> SDILGMLKSLHQLQVENRRLEEQIKNLTAKKERLQLLNAQLSV;> DWATLSLEKLLKEKQALKSQISEKQRHCL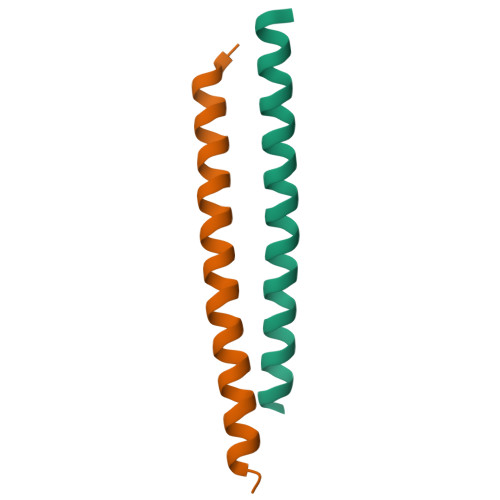ELQISIVELEK> EWTGDSSINYYSDEVISDFHVGQFNRSA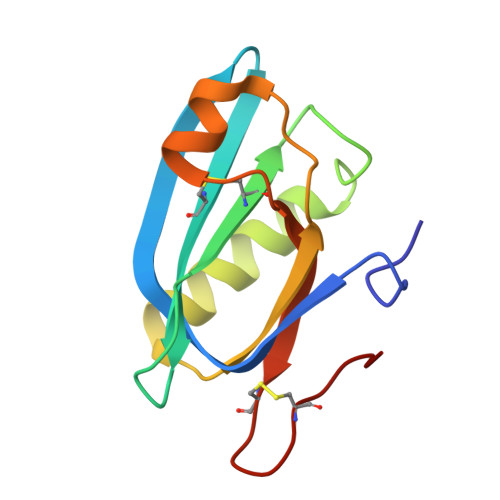YFCIKTVKKSGEGTPIIACALSHDSKWIPSFNIMLEQARNFYITGHSIRVYVQPNVWSNKSFIEALSSNALVGLSSCSTSECFGPVK>[4x]SGMKIIALRSSLKLAARIAEELKTEPVMPDERRFPDG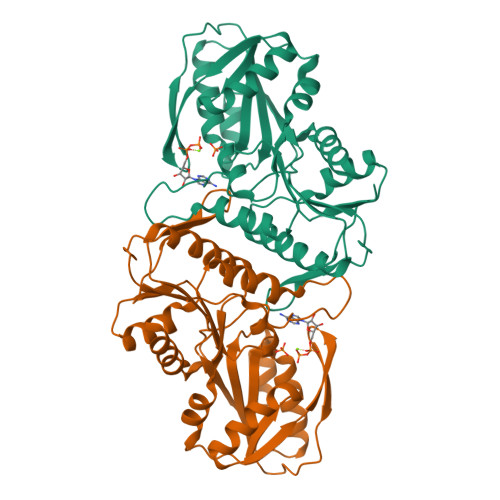ELYLRYDEDLTGHNIFIIGNTHSDAEVMEMILTLSAIQDYRTKSVNIIAPYYGYARQHQRYKNGEPISSQILTEIYSSYSNSIATVDIHDEKTLSYSKVKFSDLHANDAIVRYYKNVDVDYVVSPDDGGLARVADISAKLGKKHFFIEKKRIDDRTVEMKVPNVDVNGKKLLIVDDIISTGGTIAKSSGLLREKGASKIYVSAVHGLFVNGSENKILQNADEIHVTDTVESKFSDISVYQEVCNYIRDID>MVQVLSVLVIPLLTLFFGYVASSSIDLSVDTSEYNRPLIHFTPEKGWMNAPNGLFYDKTAKLWHLYFQYNPNATAWGQPLYWGHATSNDLV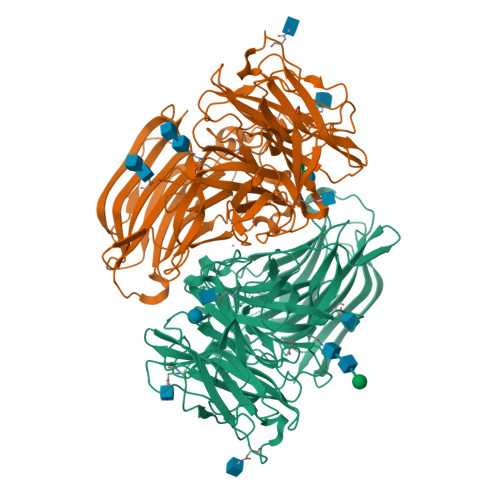HWDEHEIAIGPEHDNEGIFSGSIVVDHNNTSGFFNSSIDPNQRIVAIYTNNIPDNQTQDIAFSLDGGYTFTKYENNPVIDVSSNQFRDPKVFWHEDSNQWIMVVSKSQEYKIQIFGSANLKNWVLNSNFSSGYYGNQYECPGLIEVPIENSDKSKWVMFLAINPGSPLGGSINQYFVGDFDGFQFVPDDSQTRFVDIGKDFYAFQTFSEVEHGVLGLAWASNWQYADQVPTNPWRSSTSLARNYTLRYVHTNAETKQLTLIQNPVLPDSINVVDKLKKKNVKLTNKKPIKTNFKGSTGLFDFNITFKVLNLNVSPGKTHFDILINSQELNSSVDSIKIGFDSSQSSFYIDRHIPNVEFPRKQFFTDKLAAYLEPLDYDQDLRVFSLYGIVDKNIIELYFNDGTVAMTNTFFMGEGKYPHDIQIVTDTEEPLFELESVIIRELNK[2x]>MSVAGLKKQFHKATQKVSEKVGGAEGTKLDDDFKEMERKVDVTSRAVMEIMTKTIEYLQPNPASRAKLSMINTMSKIRGQEKGPGYPQAEALLAEAMLKFGRELGDDCNFGPALGEVGEAMRELSEVKDSLDMEVKQNFIDPLQNLHDKDLREIQHHLKKLEGRRLDFGYKK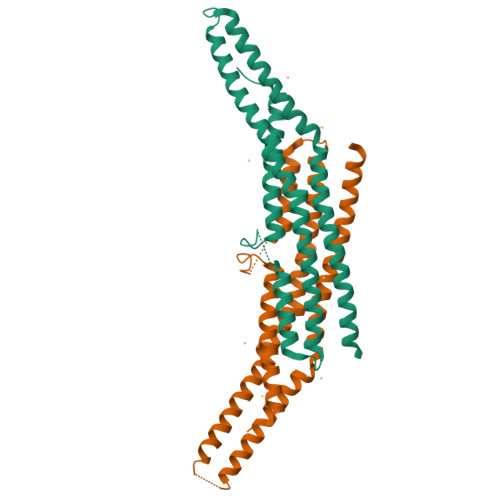KRQGKIPDEELRQALEKFDESKEIAESSMFNLLEMDIEQVSQLSALVQAQLEYHKQAVQILQQVTVRLEERIRQASSQPRREYQ[2x]>PRPHKKLKQLHWEKLDCTDNSIWGTGKAEKFADDLYEKGVLADLEKAFAAREIKSLASKEFKITFLSRDISQQFGINLHMYSSLSVADLVKKILNCDRDFLQTPSVVEFLSKSEIIEVSVNLARNYAPYSTDWEGVRNLEDAKPPEKDPNDLQRADQIYLQLMVNLESYWGSRMRALTVVTSYEREYNELLAKLRKVDKAVSALQESDNLRNVFNVILAVGNFMNDTSKQAQGFKLSTLQRLTFIKDTTNSMTFLNYVEKIVRLNYPSFNDFLSELEPVLDVVKVSIEQLVNDCKDFSQSIVNVERSVEIGNLSDSSKFHPLDKVLIKTLPVLPEARKKGDLLEDEVKLTIMEFESLMHTYGEDSGDKFAKISFFKKFADFINEYKKAQA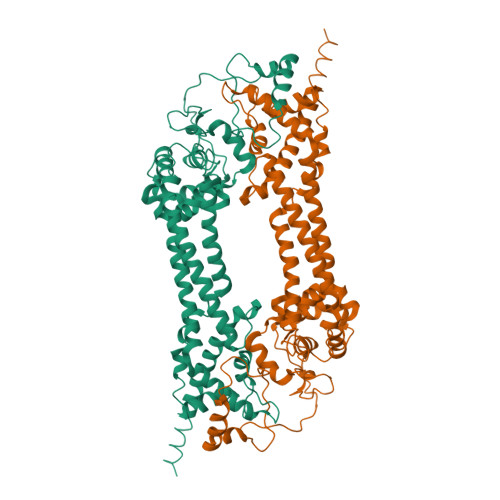QNLAAEEEERLYIKHKKIVE[2x]Methylation of cytosine 32 in the anticodon loop of tRNAs to 3-methylcytosine (m3C) is crucial for cellular translation fidelity. Here, we report the cryo-electron microscopy structure of the human m3C tRNA methyltransferase METTL6 in complex with seryl-tRNA synthetase (SerRS) and their common substrate tRNASer. We show that SerRS acts as the tRNASer substrate selection factor for METTL6. We demonstrate that SerRS augments the methylation activity of METTL6 and that direct contacts between METTL6 and SerRS are necessary for efficient tRNASer methylation.

Therefore, for the purpose of structure determination, we stabilized the assembly by fusing METTL6 to the flexible C terminus of SerRS and coexpressed both proteins as a single polypeptide in insect cells. Processing of the cryo-EM micrographs and particle images of the METTL6–SerRS–tRNASer complex revealed three-dimensional (3D) classes for 1:2:1, 1:2:2 and 2:2:2 stoichiometries with essentially identical intermolecular contacts in the METTL6–SerRS–tRNA interface. Surprisingly, despite the fusion of METTL6 to SerRS, not all of the SerRS molecules in our reconstructions displayed an associated density for METTL6. In the absence of protease treatment or cleavage sites, this suggests that the 60 amino acid-long flexible linker connecting the proteins allowed free dissociation of METTL6 and that the fusion strategy tolerated an on–off equilibrium of the assembly. In our samples, we observe different possible stoichiometries of the METTL6–SerRS–tRNA complex. In the complex with two copies of METTL6 present, these are spatially distant (~100 Å) from each other, with each METTL6 molecule binding only one tRNA, implying that that these METTL6 molecules would function independently of each other. Therefore, we would suppose that the most abundant physiological active assembly comprises the SerRS dimer, one or two tRNAs and one copy of METTL6, but does not exclude the association of a second METTL6 molecule to the complex. Mass spectrometry of the copurified tRNA confirmed the presence of m3C-modified tRNASer in our sample. In the structural model, the modified N3 atom of C32 lies at a 4 Å distance from the sulfur atom of SAH. These findings indicate that the structure captured a postcatalytic state with both products present.

>[2x]MASLQRKGLQARILTSEEEEKLKRDQTLVSDFKQQKLEQEAQKNWDLFYKRNSTNFFKDRHWTTREFEELRSCREFEDQKLTMLEAGCGVGNCLFPLLEEDPNIFAYACDFSPRAIEYVKQNPLYDTERCKVFQCDLTKDDLLDHVPPESVDVVMLIFVLSAVHPDKMHLVLQNIYKVLKPGKSVLFRDYGLYDHAMLRFKASSKLGENFYVRQDGTRSYFFTDDFLAQLFMDTGYEEVVNEYVFRETVNKKEGLCVPRVFLQSKFLKPPKNPSPVVLGLDPKS;>[2x]MVLDLDLFRVDKGGDPALIRETQEKRFKDPGLVDQLVKADSEWRRCRFRADNLNKLKNLCSKTIGEKMKKKEPVGDDESVPENVLSFDDLTADALANLKVSQIKKVRLLIDEAILKCDAERIKLEAERFENLREIGNLLHPSVPISNDEDVDNKVERIWGDCTVRKKYSHVDLVVMVDGFEGEKGAVVAGSRGYFLKGVLVFLEQALIQYALRTLGSRGYIPIYTPFFMRKEVMQEVAQLSQFDEELYKVIGKGSEKSDDNSYDEKYLIATSEQPIAALHRDEWLRPEDLPIKYAGLSTCFRQEVGSHGRDTRGIFRVHQFEKIEQFVYSSPHDNKSWEMFEEMITTAEEFYQSLGIPYHIVNIVSGSLNHAASKKLDLEAWFPGSGAFRELVSCSNCTDYQARRLRIRYGQTKKMMDKVEFVHMLNATMCATTRTICAILENYQTEKGITVPEKLKEFMPPGLQELIPFVKPAPIEQEPSKKQKKQHEGSKKKAAARDVTLENRLQNMEVTDA>[3x]PVTLEPMPPGEGAQEGEPPTVEARYKSFSIKMLKDMKEGVKQYGPNSPYMRTLLDSIAHGHRLIPYDWEILAKSSLSPSQFLQFKTWWIDGVQEQVRRNRAANPPVNIDADQLLGIGQNWSTISQQALMQNEAIEQVRAICLRAWEKIQDPGSACPSFNTVRQGSKEPYPDFVARLQDVAQKSIADEKARKVIVELMAYENANPECQSAIKPLKGKVPAGSDVISEYVKACDGIGGAMHKAMLMAQLE

CA forms the capsid shell surrounding the viral core that protects and transports the viral genome and also interacts with host cell factors that are necessary for trafficking, nuclear entry and proviral integration. Further, we assemble particles from HML2 CArec in vitro and use single-particle cryogenic electron microscopy (cryo-EM) to determine the high-resolution structures of four different types of Fullerene shell assemblies. Our studies of HML2 CArec show that an ERV retains the ability to form capsid assemblies using the same architecture as exogenous viruses. Analysis of the shell structures reveals the intra- and inter-molecular interactions that drives CA assembly into pentamers and hexamers and their association into shells that encapsidate the retroviral genome.

The largest structure is a T = 3 particle, resolved to 4.3 Å and contains a T = 1 particle within the interior, although no fixed orientation between the shells is apparent. The T = 3 shell is 300 Å in diameter and is comprised of 12 pentamers, each surrounded by five hexamers. Hexamers are located at icosahedral three-fold axes and interact across icosahedral two-fold axes. In the T = 3 particle, there are no inter-pentamer interactions, instead each pentamer is surrounded by five hexamers. The hexamers contact both pentamers and hexamers through the CTD–CTD interactions with three alternating CArec protomers linking to T = 3 pentamers and the other three linking to T = 3 hexamers. These non-equivalent contacts are accommodated by relative shifts of adjacent CA monomers reducing the hexamer to three-fold symmetry, consistent with its location at the icosahedral three-fold axis. When the CTD–CTD interaction is with a pentamer, the intra-hexamer CTD–NTD interaction has the same structural conformation and specific hydrogen bonding arrangement as the T = 1 pentamer conformation. By contrast, when the CTD–CTD interaction is with a hexamer, the CTD shifts away from its NTD by 3.6 Å, the R143-mediated α6–α7 interaction is lost and the intra-hexamer CTD–NTD interaction has a structural conformation and hydrogen-bonding configuration that is comparable to that of the D6 hexamer. Measurements of the radial distance of the centroid for T = 3 pentamers and hexamers show that pentamers are situated at a higher radius than hexamers, 143.9 and 136.5 Å, respectively. This difference in displacement is accommodated in T = 3 hexamers by the alternating shift-up of the CTDs (3.3 Å) to interact with adjacent pentamers and shift-down (3.3 Å) to interact with adjacent hexamers.>GIDPFTMTPSEDFVVTDRGGIVENSHRVHAAVVDAKGRLLYALGNPTRMTLARSAAAPAQALAILETEGVAGYGFDDADIALMCASHSSEDRHIARTRAMLSKIKAEEADLRCGGHPSLSEMVNRSWIKQDFIPTAVCSNCSGKHVGMLAGARAIGAGTDGYHLPDHPMQGRVKRTVAELCDLDAGDVEWGTDGCNLPTPAFPLDRLGRIYAKLASAADGSDAGEGQSTRCAALAHIFRAMARYPEMVAGEGRYCTMLMRAFDGALVGKLGADASYAIGVRASDATRQLGTDGALGISVKIEDGNLEMLYAVVTELLERLGIGSPDVRSQLASFHHPQRVNTMGVTTGGVSFPFKLRGSKSNVDDPRLAAVAR[2x]

The ReAV enzyme from Rhizobium etli, a representative of Class 3 L-asparaginases, is sequentially and structurally different from other known L-asparaginases. Asparaginases (EC 3.5.1.1) catalyze the hydrolysis of L-asparagine, generating L-aspartate and ammonia. ReAV is a homodimeric protein, with each subunit containing a highly specific zinc-binding site created by two cysteines, a lysine, and a water molecule. Two Ser-Lys tandems (Ser48-Lys51, Ser80-Lys263) are located in the close proximity of the metal binding site, with Ser48 hypothesized to be the catalytic nucleophile.

Substitution of Lys51 with alanine induced notable structural rearrangements within the active site region, and these changes are not strictly equivalent in the two protein chains. In chain A, the absence of Lys51 affects the position and conformational state of Lys138 in the metal coordination sphere. The side chain of Lys138 adopts two alternative conformations: one rotamer moves away from the metal cation and forms H-bonds with the Oε atom of Gln54 and the Oγ atom of Ser48, while the other rotamer maintains its typical conformation, pointing toward the Zn2+ cation. Furthermore, both the zinc cation and the coordinated water molecule are only partially present in the mutant crystal structure, with a refined occupancy of 0.5. The Ser48 side chain has a slightly different position depending on the protein chain, without the characteristic pattern of three closely spaced water molecules. In protein chain B, Ser48 retains its typical conformation, pointing toward the water molecule in the metal coordination sphere; however, the interaction with the Oγ atom of Ser80 is no longer possible. As observed in the previously described S48A mutant structure, a sulfate ion (at 0.5 occupancy) from the crystallization solution appears in the active site area, forming H-bonds with the Nη atom of Arg47, the main-chain N atoms of Gly188 and Cys189, and one or more water molecules, depending on the protein chain. Structural analysis and careful inspection of the electron density maps revealed the presence of an unintended, second mutation at position 238, where His was expected. Thus, the crystal structure of the K51A mutant discussed in this work actually corresponds to the double K51A/H238Y mutant. The Lys51 residue from the Ser48-Lys51 tandem, with its side chain unprotonated at the high pH (9.0) of the catalytic reaction, acts as a base for proton abstraction from Ser48 and participates in the proton shuttling network during the catalytic process. The K51A mutein is incapable of L-asparagine hydrolysis because the Lys51 side chain can no longer play the role of the nucleophilic activator.>SKKQDENIVVNKFKPKEPYVGRCLLNTKITGDDAPGETWHMVFSTEGEVPYREGQSIGIVPDGIDKNGKPHKLRLYSIASSAIGDFGDSKTVSLCVKRLVYTNDAGEVVKGVCSNFLCDLKPGSEVKITGPVGKEMLMPKDPNATVIMLGTGTGIAPFRSFLWKMFFEKHEDYQFNGLAWLFLGVPTSSSLLYKEEFEKMKEKAPENFRLDFAVSREQVNDKGEKMYIQTRMAQYAEELWELLKKDNTFVYMCGLKGMEKGIDDIM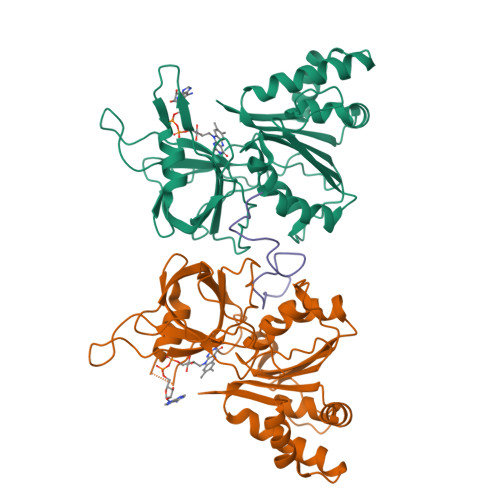VSLAAKDGIDWIEYKRTLKKAEQWNVEVYL[2x];> KTEQPLSPYTAYDDLKPPSSPSPTKP> TILRRSRSDR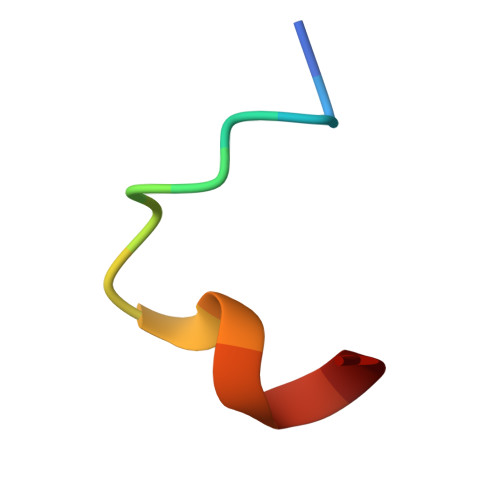KKLA>MFPEVVELNVGGQVYFTRHSTLISIPHSL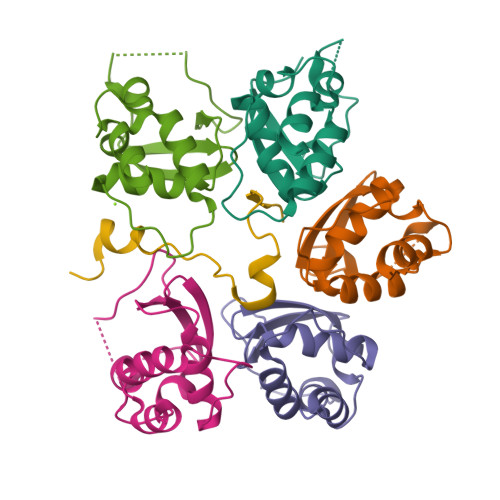LWKMFSPKRDTANDLAKDSKGRFFIDRDGFLFRYILDYLRDRQVVLPDHFPEKGRLKREAEYFQLPDLVKLLTP[10x];>[2x]GPEKDPIEDINSPEHIQRRLSLQLPILHHAYLPSIGGVDAS> XSLSAAEADLAGKSWAPVFANKNANGLDFLVALFEKFPDSANFFADFKGKSVADIKASPKLRDVSSRIFTRLNEFVNNAANAGKMSAMLSQFAKEHVGFGVGSAQFE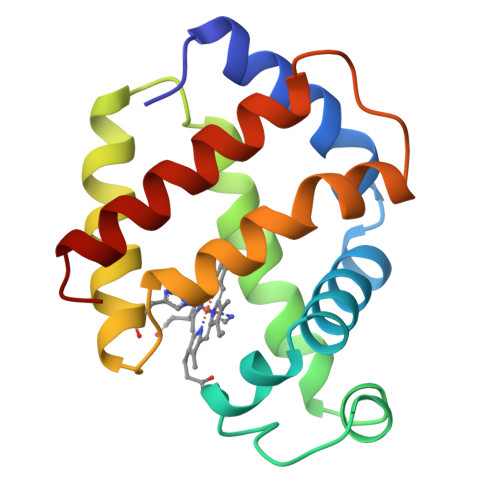NVRSMFPGFVASVAAPPAGADAAWTKLFGLIIDALKAAGA> MSDLFLELNGKVHSLSETFPGLSVQEVSRQSPQ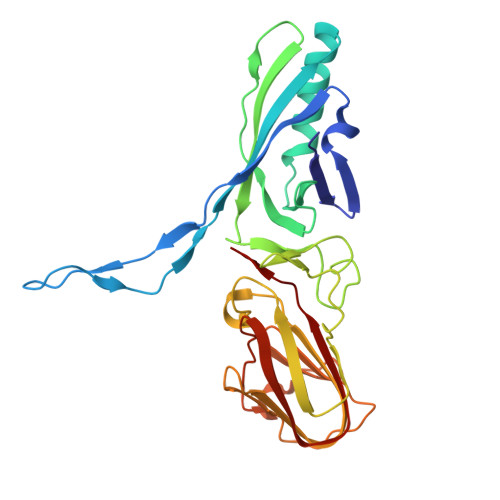LSMETAEIAGTDGVIPGMTQFKPFIFSAKCNLQALDIPDYHLAVREIYEFLFQRDSYYIWSDQMPGIRYEVHPKPVDFSRESDRVGLLTIEFDVFKGYAESRGTSLDPMTFEVDLWQMGMNLSNRDDLFYVFRENTFRVYNAGSDRVNPLMRHELDIAMTANGTPTIHNLTTGESFEYRKELQKTDVLLLNNIYPLVNNRRVGKDTNHGIITLEKGWNDFEIKGVTDVTIAFNFPFIYR>SNAMSTDRESQLLRQATKAGIDSPLELANFMAQAGHESRGLSRLNESFNFTRGISQIPVEAAWRNGNAALESARQEALRGRPENLAELMYGGRMGNDAPGDALKYHGRGYLPLVGKENYERAGKALDLDLVNQPELAAQPEHAGRIAVWQWQTRVPEGARHDVREATYALNGALNGIEARRQR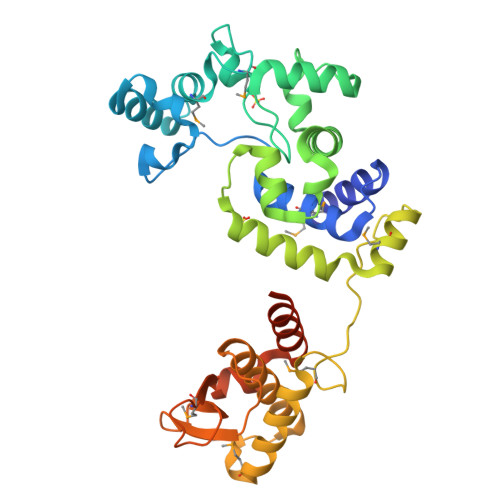FEVWQQKLTPDVMARLDRGEVGAPAQTVARDMSHAGEPGNALFEDARQHLRQMGPQSGLRSAQELDNTAGALALGAQKAGLSRIDHLLAGNDGRTLFAVQGALGDPAMLRASVDREQASQQSLAQSSQQLAASVAQQDPTAALAREQEQRSRSL[2x]>RTFDLEEKLQTNKYNANFVTFMEGKDFNVEYIQRGGLRDPLIFKNSDGLGIKMPDPDFTVNDVKMCVGSRRMVDVMDVNTQKGIEMTMAQWTRYYETPEEEREKLYNVISLEFSHTRLENMVQRPSTVDFIDWVDNMWPRHLKESQTESTNAILEMQYPKVQKYCLMSVRGCYTDFHVDFGGTSVWYHIHQGGKVFWLIPPTAHNLELYENWLLSGKQGDIFLGDRVSDCQRIELKQGYTFVIPSGWIHAVYTPTDTLVFGGNFLHSFNIPMQLKIYSIEDRTRVPNKFRYPFYYEMCWYVLERYVYCITNRSHLTKDFQKESLSMDME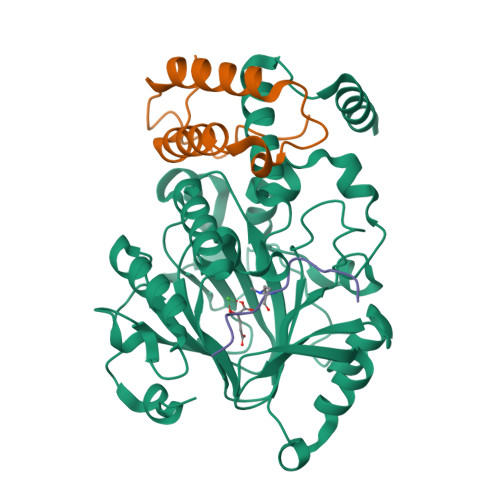[2x];>QVHLTHFELEGLRCLVDKLESLPLHKKCVPTGIEDEDALIADVKILLEELASSDPKLALTGVPIVQWP[2x];>[2x]APATGGVKKPHRYRP>[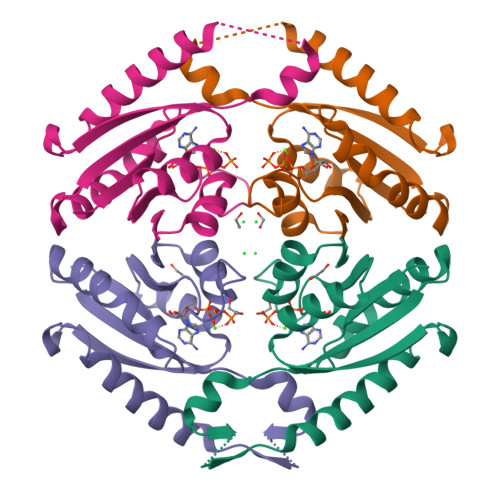2x]MRGSHHHHHHGMASMNRTILVPIDISDSELTQRVISHVEAEAKIDDAKVHFLTVIPSLPYYASLGLAYSAELPAMDDLKAEAKSQLEAIIKKFNLPADRVQAHVAEGSPKDKILEMAKKLPADMVIIASHRPDITTYLLGSNAAAVVRHAECSVLVVR> MKIEEGKVVIWHAMQPNELEVFQSLAEEYMALCPEVEIVFEQKPNLEDALKAAI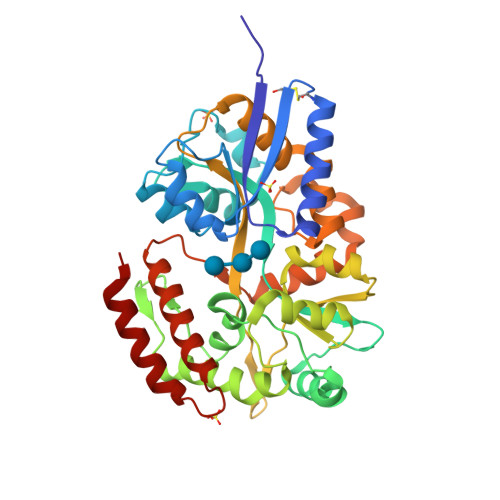PTGQGPDLFIWAHDWIGKFAEAGLLEPIDEYVTEDLLNEFAPMAQDAMQYKGHYYALPFAAETVAIIYNKEMVSEPPKTFDEMKAIMEKYYDPANEKYGIAWPINAYFISAIAQAFGGYYFDDKTEQPGLDKPETIEGFKFFFTEIWPYMAPTGDYNTQQSIFLEGRAPMMVNGPWSINDVKKAGINFGVVPLPPIIKDGKEYWPRPYGGVKLIYFAAGIKNKDAAWKFAKWLTTSEESIKTLALELGYIPVLTKVLDDPEIKNDPVIYGFGQAVQHAYLMPKSPKMSAVWGGVDGAINEILQDPQNADIEGILKKYQQEILNNMQG>[2x]MGSTEYKPTVRLATRDDVPRAVRTLAAAFADYPATRHTVDPDRHIERVT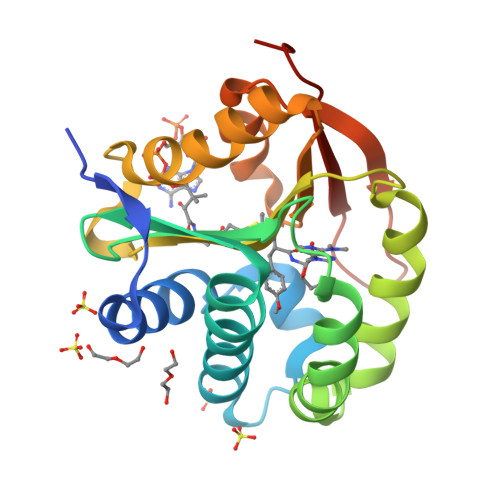ELQELFLTRVGLDIGKVWVADDGAAVAVWTTPESVEAGAVFAEIGPRMAELSGSRLAAQQQMEGLLAPHRPKEPAWFLATVGVSPDHQGKGLGSAVVLPGVEAAERAGVPAFLETSAPRNLPFYERLGFTVTADVEVPEGPRTWCMTRKPGASHHHHHH> MADLKAAEVEKAREHFEIYDWEGEGKIDARDLGDLLRSLDCKPTLAMVKKNGGSDKRG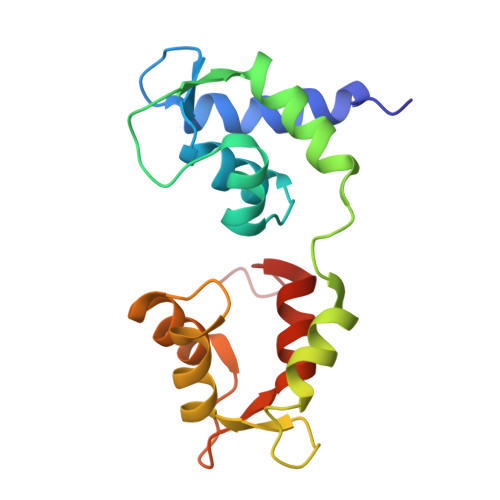EKKLTLEEFLPIFSQIKKEKEVGTLEDFMEGLKVYDKAENGTMLAAELAHVLLSLGERLTDIECEEIMRVCDEDDDGFLKYEPFVKTIIAGPFPDEGK> MEQKPGTLMVYVVVGYNTDNTVDVVGGAQYAVSPYLFLDVGYGWNNSSLNFLEVGGGVSYKVSPDLEPYVKAGFEYNTDNTIKPTAGAGALYRVSPNLALMV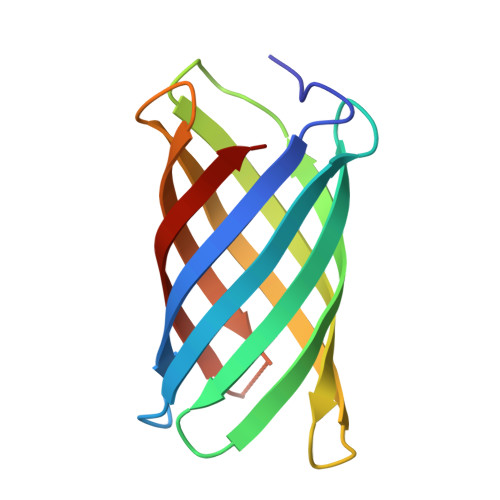EYGWNNSSLQKVAIGIAYKVKD>[2x]PQSEARRRILETAWRLIARRGYHNVRIHDIASELGTSNATIHYHFPSKKDILLEALRRNVKLAFDRQVA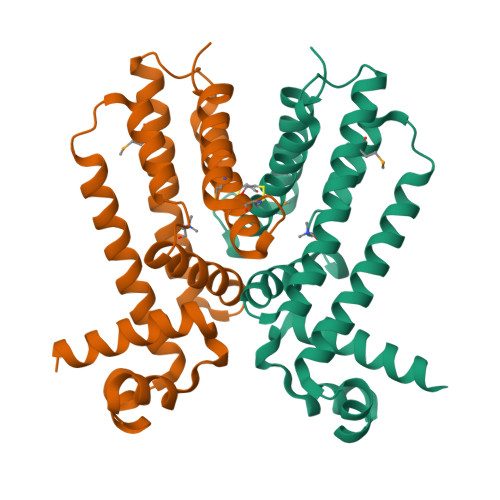ELHTIADARERLVRLVELQLPTPGLLRDEWSVWLQVWTESTLNPKIRDLYNDAYDRWYQTIAMTIRTGQKQGVFRDQDADELATRLSALIDGLGIQVLTGKRGCSVDHMRQHLNDFIEHNIVERRP> MKLTIHEIAQVVGAKNDISIFEDTQLEKAEFDSRLIGTGDLFVPLKGARDGHDFIETAFENGAAVTLSEKEVSNHPYILVDDVLTAFQSLASYYLEKTTVDVFAVTGSNGKTTTKDMLAHLLSTRYKTYKTQGNYNNEIGLPYTVLHMPEGTEKLVLEMGQDHLGDIHLLSELARPKTAIVTLVGEAHLAFFKDRSEIAKGKMQIADGMASGSLLLAPADPIVEDYLPIDKKVVRFGQGAELEITDLVERKDS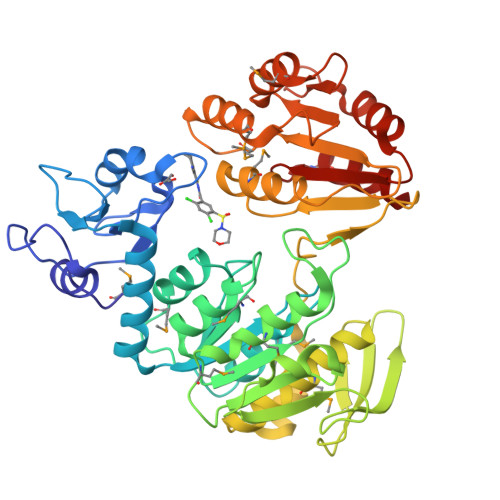LTFKANFLEQALDLPVTGKYNATNAMIASYVALQEGVSEEQIRLAFQHLELTRNRTEWKKAANGADILSDVYNANPTAMKLILETFSAIPANEGGKKIAVLADMKELGDQSVQLHNQMILSLSPDVLDIVIFYGEDIAQLAQLASQMFPIGHVYYFKKTEDQDQFEDLVKQVKESLGAHDQILLKGSNSMNLAKLVESLEN>MRSIIKGRVWKFGNNVDTDAILPARYLVYTKPEELAQFVMTGADPDFPKKVKPGDIIVGGKNFGCGSSREHAPLGLKGAGISCVIAESFARIFYRNAINVGLPLIECKGISEKVNEGDELEVNLETGEIKNLTTGEVLKGQKLPEFMMEILEAGGLMPYLKKKMA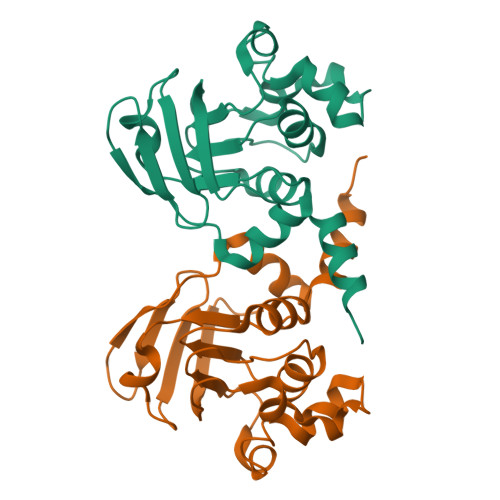ESQLEHHHHHH[6x]> MTNESILESYSGVTPERKKSRMPAKLDWWQSATGLFLGLFMIGHMFFVSTILLGDNVMLWVTKKFELDFIFEGGKPIVVSFLAAFVFAVFIAHAFLAMRKFPINYRQYLTFKTHKDLMRHGDTTLWWIQAMTGFAMFFLGSVHLYIMMTQPQTIGPVSSSFRMVSEWMWPLYLVLLFAVQ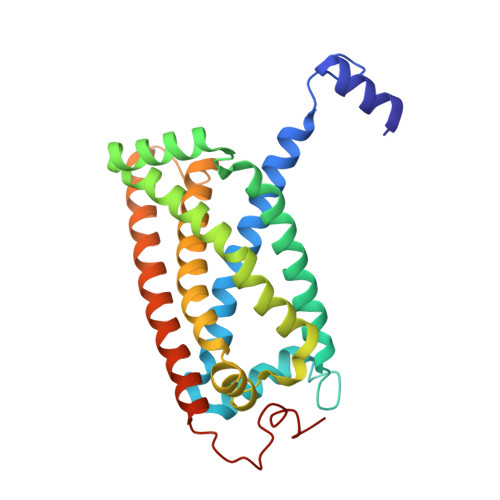LHGSVGLYRLAVKWGWFDGETPDKTRANLKKLKTLMSAFLIVLGLLTFGAYVKKGLEQTDPNIDYKYFDYKRTHHR> MGSDYKDHDGDYKDHDIDYKDDDDKGSGSLEVLFQGPMDPLNESTVNVYLPDSYLKGVISFSETNAIGSCLLKRPYLKNDNTAKVAIENPVIEHVRLKNAVNSKMKISDYKVVEPVNMQHEIMKNVHSCELTLLKQFLTRSKNISTLKLNMICDWLQLKSTSDDTSILSFIDVEFIPSWVSNWFSNWYNLNKLILEFRREEVIRTGSILCRSLGKLVFIVSSYGCIVKSNKSKRVSFFTYNQLLTWKDVMLSRFNANFCIWVSNSLNENQEGLGLRSNLQGMLTNKLYETVDYMLSLCCNEGFSLVKEFEGFIMSEILRITEHAQFSTRFRNTLLNGLTDQLTKLKNKNRLRVHSTVLENNDYPMYEVVLKLLGDTLRCIKLLINKNLENAAELYYIFRIFGHPMVDERDAMDAVKLNNEITKILRLESLTELRGAFILRIIKGFVDNNKRWPKIKNLKVLSKRWTMYFKAKNYPSQLELSEQDFLELAAIQFEQEFSVPEKTNLEMVLNDKAISPPKRLIWSVYPKNYLPETIKNRYLEETFNASDSLKTRRVLEYYLKDNKFDQKELKSYVVRQEYLNDKEHIVSLTGKERELSVGRMFAMQPGKQRQIQILAEKLLADNIVPFFPETLTKYGDLDLQRIMEIKSELSSIKTRRNDSYNNYIARASIVTDLSKFNQAFRYETTAICADVADELHGTQSLFCWLHLIVPMTTMICAYRHAPPETKGEYDIDKIEEQSGLYRYHMGGIEGWCQKLWTMEAISLLDVVSVKTRCQMTSLLNGDNQSIDVSKPVKLSEGLDEVKADYRLAVKMLKEIRDAYRNIGHKLKEGETYISRDLQFISKVIQSEGVMHPTPIKKVLRVGPWINTILDDIKTSAESIGSLCQELEFRGESIIVSLILRNFWLYNLYMHESKQHPLAGKQLFKQLNKTLTSVQRFFEIKRENEVVDLWMNIPMQFGGGDPVVFYRSFYRRTPDFLTEAISHVDILLKISANIKNETKVSFFKALLSIEKNERATLTTLMRDPQAVGSERQAKVTSDINRTAVTSILSLSPNQLFSDSAIHYSRNEEEVGIIAENITPVYPHGLRVLYESLPFHKAEKVVNMISGTKSITNLLQRTSAINGEDIDRAVSMMLENLGLLSRILSVVVDSIEIPIKSNGRLICCQISRTLRETSWNNMEIVGVTSPSITTCMDVIYATSSHLKGIIIEKFSTDRTTRGQRGPKSPWVGSSTQEKKLVPVYNRQILSKQQREQLEAIGKMRWVYKGTPGLRRLLNKICLGSLGISYKCVKPLLPRFMSVNFLHRLSVSSRPMEFPASVPAYRTTNYHFDTSPINQALSERFGNEDINLVFQNAISCGISIMSVVEQLTGRSPKQLVLIPQLEEIDIMPPPVFQGKFNYKLVDKITSDQHIFSPDKIDMLTLGKMLMPTIKGQKTDQFLNKRENYFHGNNLIESLSAALACHWCGILTEQCIENNIFKKDWGDGFISDHAFMDFKIFLCVFKTKLLCSWGSQGKNIKDEDIVDESIDKLLRIDNTFWRMFSKVMFEPKVKKRIMLYDVKFLSLVGYIGFKNWFIEQLRSAELHEIPWIVNAEGDLVEIKSIKIYLQLIEQSLFLRITVLNYTDMAHALTRLIRKKLMCDNALLTPISSPMVNLTQVIDPTTQLDYFPKITFERLKNYDTSSNYAKGKLTRNYMILLPWQHVNRYNFVFSSTGCKVSLKTCIGKLMKDLNPKVLYFIGEGAGNWMARTACEYPDIKFVYRSLKDDLDHHYPLEYQRVIGELSRIIDSGEGLSMETTDATQKTHWDLIHRVSKDALLITLCDAEFKDRDDFFKMVILWRKHVLSCRICTTYGTDLYLFAKYHAKDCNVKLPFFVRSVATFIMQGSKLSGSECYILLTLGHHNSLPCHGEIQNSKMKIAVCNDFYAAKKLDNKSIEANCKSLLSGLRIPINKKELDRQRRLLTLQSNHSSVATVGGSKIIESKWLTNKASTIIDWLEHILNSPKGELNYDFFEALENTYPNMIKLIDNLGNAEIKKLIKVTGYMLVSKK;>[4x]MSFPEGKDILFMGNEAAKLAEAFQKSLRKPSHKRSQSIIGEKVNTVSETLELPTISRPTKPTILSEPKLAWTDKGGAIKTEAKQTIKVMDPIEEEEFTEKRVLPSSDGKTPAEKKLKPSTNTKKKVSFTPNEPGKYTKLEKDALDLLSDNEEEDAESSILTFEERDTSSLSIEARLESIEEKLSMILGLLRTLNIATAGPTAARDGIRDAMIGIREELIADIIKEAKGKAAEMMEEEMNQRTKIGNGSVKLTEKAKELNKIVEDESTSGESEEEEELKDTQENNQEDDIYQLIMKGENKYFQGHHHHHHH

The polymerase is a multifunctional enzyme that is responsible for transcribing the viral negative sense RNA genome to generate polyadenylated mRNAs with a 5′ methylguanosine cap and replicating it to generate new viral genomes. The L protein contains three enzymatic domains: an RNA-dependent RNA polymerase (RdRp), a polyribonucleotidyltransferase (PRNTase), which is involved in cap addition, and a methyltransferase (MTase) that methylates the cap. Here we report a conserved allosteric inhibitory site identified on the L polymerase proteins of RSV and HMPV that can be targeted by a dual-specificity, non-nucleoside inhibitor, termed MRK-1. Functional analyses indicate that MRK-1 inhibits conformational changes necessary for the polymerase to engage in RNA synthesis initiation and to transition into an elongation mode.

To compare the binding of MRK-1 to HMPV L with that of RSV L, full-length HMPV L-P complexes were purified and the structure of the MRK-1 liganded HMPV L-P structure was solved at a resolution of 2.74 Å. The structure of MRK-1-bound HMPV “L” chain Cα backbone superposes over that of the apo enzyme with a r.m.s.d. of 1.1 Å for 1204 atoms, indicating that the structures are similar. The inhibitor binds in the groove present on the PRNTase domain next to the catalytic His1263 residue, equivalent to the RSV binding site, mimicking the same binding pose. In addition, the HMPV polymerase structure undergoes similar local structural rearrangements upon complexation with the ligand, namely re-orientation of the HMPV L His1263, Arg1264, and Phe1310 side chains that correspond to RSV L His1338, Arg1339, and Phe1385. Hence the MRK-1-liganded RSV and HMPV structures are highly similar with each other, explaining why MRK-1 has antiviral activities against both viruses. However, a structural rationale for these differences may be based on the lone sequence mismatch among amino acids with their side chains pointing toward the ligand between the polymerases’ MRK-1 binding sites; specifically, RSV Cys1388 analogous to HMPV Ala1313. The RSV Cys1388 side chain sulfur mediates favorable interactions with the fluorophenyl (closest distance to phenyl 4.05 Å) of MRK-1. The contact is missing in HMPV with substitution to Ala. Instead, an empty space is present between the alanine and the inhibitor (closest distance to phenyl 4.82 Å), which could be filled with a water molecule that would be in an unfavorable hydrophobic environment. Thus, the cryo-EM structures of the MRK-1 liganded RSV and HMPV polymerases provide insight into how the compound has broad spectrum inhibition of RSV and HMPV, while also suggesting why it has lower potency against HMPV.N-(AMINOCARBONYL)-BETA-ALANINE | C4 H8 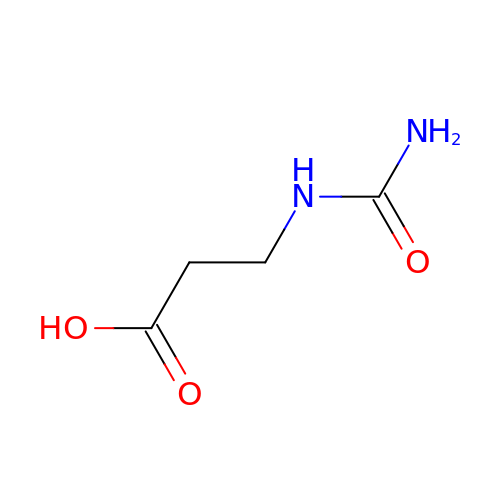N2 O3 | JSJWCHRYRHKBBW-UHFFFAOYSA-N>[2x]CC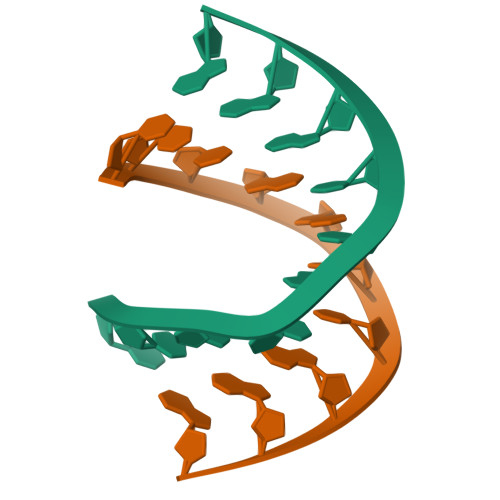CGGCCGGG9-AMINO-2-DEOXY-2,3-DEHYDRO-N-ACETYL-NEURAMINIC 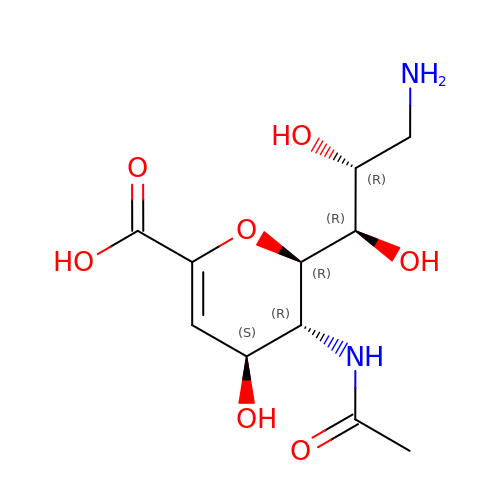ACID | C11 H18 N2 O7 | VJTPBNUXDULDQD-UFGQHTETSA-N>[2x]MRGVFLDKDKIPYDLVTKKLNEWYTSIKNDQVEQAEIIKTEVEKELLNMEENQDALLYYQLLEFRHEIMLSYMKSKEIEDLNNAYETIKEIEKQGQLTGMLEYYFYFFKGMYEFRRKELISAISAYRIAESKLSEVEDEIEKAEFFFKVSYVYYYMKQTYFSMNYANRALKIFREYEEYAVQTVRCQFIVAGNLIDSLEYERALEQFLKSLEISKESNIEHLIAMSHMNIGICYDELKEYKKASQ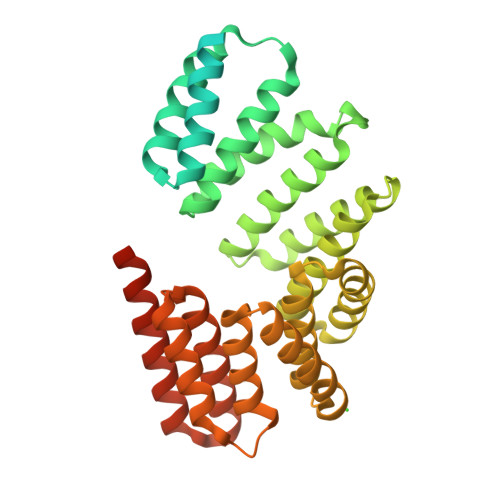HLILALEIFEKSKHSFLTKTLFTLTYVEAKQQNYNVALIYFRKGRFIADKSDDKEYSAKFKILEGLFFSDGETQLIKNAFSYLASRKMFADVENFSIEVADYFHEQGNLMLSNEYYRMSIEARRKIKKGEIIDENQPDSIGSSDFK> MATTTVGLTDLKVRLVRDDFADAVAWVARSLPSRPTVPVLAGVLLTGSDDGLTISSFDYEVSAEVQIPAEIAAPGTVLVSGRLLSEITRALPNKPVDLSVEGTRVSLTCGSARFSLPTMAVEDYPALPELPAETGSVPADLFAEA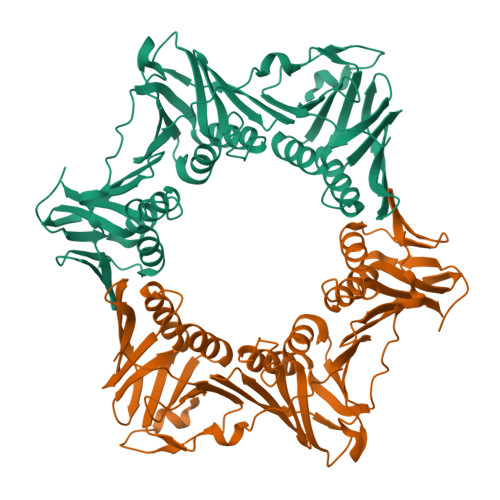IGQVAVAAGRDDTLPMLTGIRVEISGDRMVLAATDRFRLAVRELTWTTKTPDVEAAVLVPAKTLAEAAKTGLDGSEVQLALGAGPSVGQDGLLGIRSEGKRSTTRLLDAEFPKFRQLLPTEHTAMATIGVGELTEAIKRVALVADRGAQVRMEFADDVLHLSAGADDVGRAEEDLPVSFSGEPLTIAFNPGYLTDGLGALHSERVTFGFTTPSKPAVLRPATEADAALNGNGPFPAAETDYVYLLMPVRLPG>MKILVIEDDALLLQGLILAMQSEGYVCDGVSTAHEAALSLASNHYSLIVLDLGLPDEDGLHFLSRM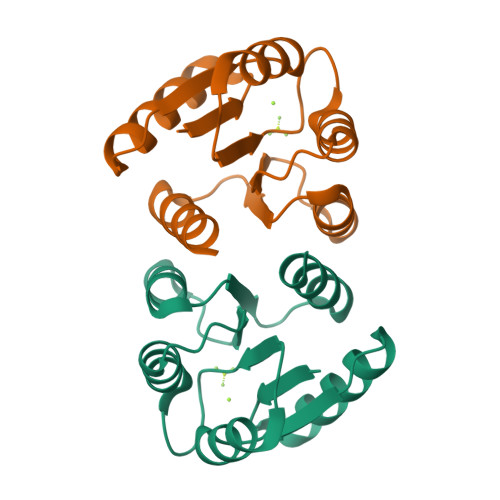RREKMTQPVLILTARDTLEDRISGLDTGADDYLVKPFALEELNARIRALLRRHNNQGLEHHHHHH[2x]> TVTKVSLPEGSFKRVKPQYDEIHIPAPSKPVIDYELKEITSLPDWCQEAFPSSETTSLNPIQSKVFHAAFEGDSNMLICAPTGSGKTNIALLTVLKALSHHYNPKTKKLNLSAFKIVYIAPLKALVQEQVREFQRRLAFLGIKVAELTGDSRLSRKQIDETQVLVSTPEKWDITTRNSNNLAIVELVRLLIIDEIHLLHDDRGPVLESIVARTFWASKYGQEYPRIIGLSATLPNYEDVGRFLRVPKEGLFYFDSSFRPCPLSQQFCGIKERNSLKKLKAMNDACYEKVLESINEGNQIIVFVHSRKETSRTATWLKNKFAEENITHKLTKNDAGSKQILKTEAANVLDPSLRKLIESGIGTHHAGLTRSDRSLSEDLFADGLLQVLVCTATLAWGVNLPAHTVIIKGTDVYSPEKGSWEQLSPQDVLQMLGRAGRPRYDTFGEGIIITDQSNVQYYLSVLNQQLPIESQFVSKLVDNLNAEVVAGNIKCRNDAVNWLAYTYLYVRMLASPMLYKVPDISSDGQLKKFRESLVHSALCILKEQELVLYDAENDVIEATDLGNIASSFYINHASMDVYNRELDEHTTQIDLFRIFSMSEEFKYVSVRYEEKRELKQLLEKAPIPIREDIDDPLAKVNVLLQSYFSQLKFEGFALNSDIVFIHQNAGRLLRAMFEICLKRGWGHPTRMLLNLCKSATTKMWPTNCPLRQFKTCPVEVIKRLEASTVPWGDYLQLETPAEVGRAIRSEKYGKQVYDLLKRFPKMSVTCNAQPITRSVMRFNIEIIADWIWDMNVHGSLEPFLLMLEDTDGDSILYYDVLFITPDIVGHEFTLSFTYELKQHNQNNLPPNFFLTLISENWWHSEFEIPVSFNGFKLPKKFPPPTPLLENISISTSELGNDDFSEVFEFKTFNKIQSQVFESLYNSNDSVFVGSGKGTGKTAMAELALLNHWRQNKGRAVYINPSGEKIDFLLSDWNKRFSHLAGGKIINKLGNDPSLNLKLLAKSHVLLATPVQFELLSRRWRQRKNIQSLELMIYDDAHEISQGVYGAVYETLISRMIFIATQLEKKIRFVCLSNCLANARDFGEWAGMTKSNIYNFSPSERIEPLEINIQSFKDVEHISFNFSMLQMAFEASAAAAGNRNSSSVFLPSRKDCMEVASAFMKFSKAIEWDMLNVEEEQIVPYIEKLTDGHLRAPLKHGVGILYKGMASNDERIVKRLYEYGAVSVLLISKDCSAFACKTDEVIILGTNLYDGAEHKYMPYTINELLEMVGLASGNDSMAGKVLILTSHNMKAYYKKFLIEPLPTESYLQYIIHDTLNNEIANSIIQSKQDCVDWFTYSYFYRRIHVNPSYYGVRDTSPHGISVFLSNLVETCLNDLVESSFIEIDDTEAEVTAEVNGGDDEATEIISTLSNGLIASHYGVSFFTIQSFVSSLSNTSTLKNMLYVLSTAVEFESVPLRKGDRALLVKLSKRLPLRFPEHTSSGSVSFKVFLLLQAYFSRLELPVDFQNDLKDILEKVVPLINVVVDILSANGYLNATTAMDLAQMLIQGVWDVDNPLRQIPHFNNKILEKCKEINVETVYDIMALEDEERDEILTLTDSQLAQVAAFVNNYPNVELTYSLNNSDSLISGVKQKITIQLTRDVEPENLQVTSEKYPFDKLESWWLVLGEVSKKELYAIKKVTLNKETQQYELEFDTPTSGKHNLTIWCVCDSYLDADKELSFEINVK;> SKNEWRKS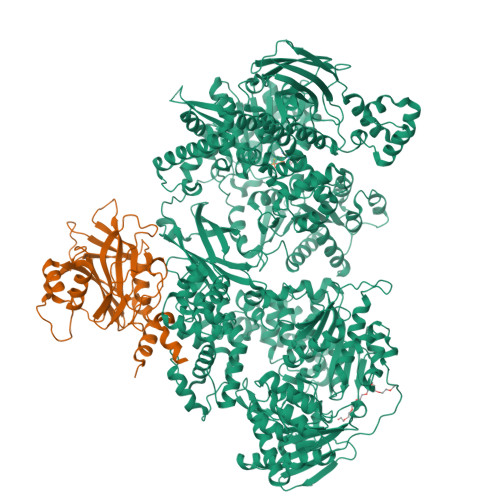AIANTLLYLRLKNIYVSADDFVEEQNVYVLPKNLLKKFIEISDVKIQVAAFIYGMSAKDHPKVKEIKTVVLVPQLGHVGSVQISNIPDIGDLPDTEGLELLGWIHTQTEELKFMAASEVATHSKLFADKKRDCIDISIFSTPGSVSLSAYNLTDEGYQWGEENKDIMNVLSEGFEPTFSTHAQLLLSDRITGNFIIPSGNVWNYTFMGTAFNQEGDYNFKYGIPLEFYNEMHRPVHFLQF>[2x]MLRKDIGIDLGTANTLVFLRGKGIVVNEPSVIAI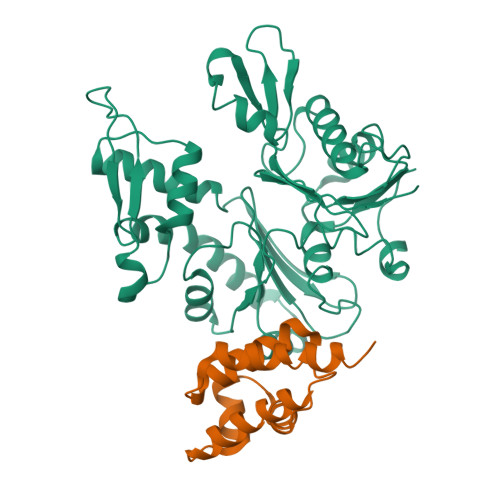DSTTGEILKVGLEAKNMIGKTPATIKAIRPMRDGVIADYTVALVMLRYFINKAKGGMNLFKPRVVIGVPIGITDVERRAILDAGLEAGASKVFLIEEPMAAAIGSNLNVEEPSGNMVVDIGGGTTEVAVISLGSIVTWESIRIAGDEMDEAIVQYVRETYRVAIGERTAERVKIEIGNVFPSKENDELETTVSGIDLSTGLPRKLTLKGGEVREALRSVVVAIVESVRTTLEKTPPELVSDIIERGIFLTGGGSLLRGLDTLLQKETGISVIRSEEPLTAVAKGAGMVLDKVNILKKLQGAGGSHHHHHH;>MSEKWKELGETFRKKREERRITLLDASLFTNINPSKLKRIEEGDLKGLDAEVYIKSYIKRYSEFLELSPDEMLKLYEEGKEEVAEEVEEKKPRKKKEKEKTRDLGSHHHHHH[2x]> MWIIEAEGDILKGKSRILFPGTYIVGRNVSDDSSHIQVISKSISKRHARFTILTPSEKDYFTGGPCEFEVKDLDTKFGTKVNEKVVGQNGDS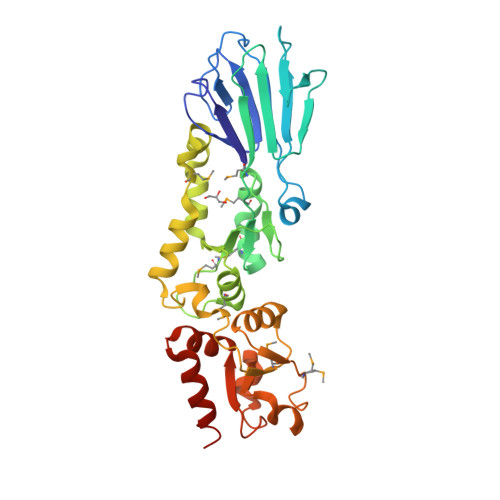YKEKDLKIQLGKCPFTINAYWRSMCIQFDNPEMLSQWASNLNLLGIPTGLRDSDATTHFVMNRQAGSSITVGTMYAFLKKTVIIDDSYLQYLSTVKESVIEDASLMPDALECFKNIIKNNDQFPSSPEDCINSLEGFSCAMLNTSSESHHLLELLGLRISTFMSLGDIDKELISKTDFVVLNNAVYDSEKISFPEGIFCLTIEQLWKIIIERNSRELISKEIERLKYATASN>[2x]SNAPDVIRLDSMSLFDTGKWVLKPGSTKRL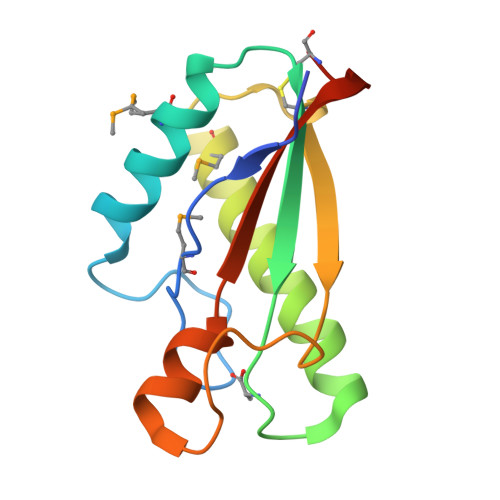VSSLMDIKARPGWLIVVAGHTDSVGEEKANQLLSLKRAESVRDWMRDTGDVPDSCFAVQGYGESRPIATNDTPEGRALNRRVEISLVPQVDACRLPD> MAGLATIDELQTLMSTVFEDDALEQAQLVLDIVSSWARVVSGQMWPDAPANVPDDVRAVVL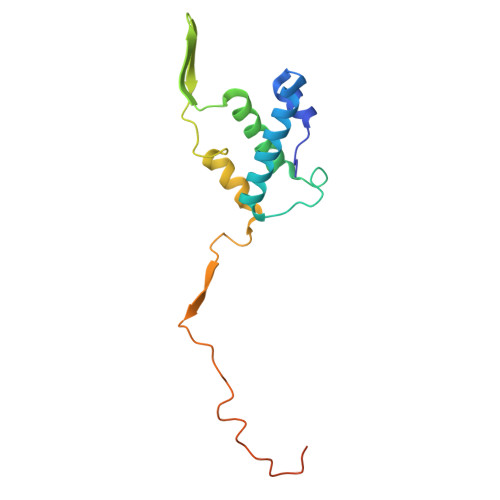QASRRELKNPDRVISRQMGPFNVQYSQPPDGFFYPAELAILKRFKRSGGLMTVSTSRGEEGRPWAGKTAYIRYGDGLFPFCSEDEGYGDVVPW> HHHHHHVPYSSAQSTSKTSVTLSLGGGTHADSLNNLANIKREQGNIEEAVRLYRKALEVFPEFAAAHSNLASVLQQQGKLQEALMHYKEAIRISPTFADAYSNMGNTLKEMQDVQGALQCYTRAIQINPAFADAHSNLASIHKDSGNIPEAIASYRTALKLKPDFPDAYCNLAHCLQIVCDWTDYDERMKKLVSIVADQLEKNRLPSVHPHHSMLYPLSHGFRKAIAERHGNLCLDKINVLHKPPYEHPKDLKLSDGRLRVGYVSSDFGNHPTSHLMQSIPGMHNPDKFEVFCYALSPDDGTNFRVKVMAEANHFIDLSQIPCNGKAADRIHQDGIHILVNMNGYTKGARNELFALRPAPIQAMWLGYPGTSGALFMDYIITDQETSPAEVAEQYSEKLAYMPHTFFIGDHANMFPHLKKKAVIDFKSNGHIYDNRIVLNGIDLKAFLDSLPDVKIVKMKCPDGGDNADSSNTALNMPVIPMNTIAEAVIEMINRGQIQITINGFSISNGLATTQINNKAATGEEVPRTIIVTTRSQYGLPEDAIVYCNFNQLYKIDPSTLQMWANILKRVPNSVLWLLRFPAVGE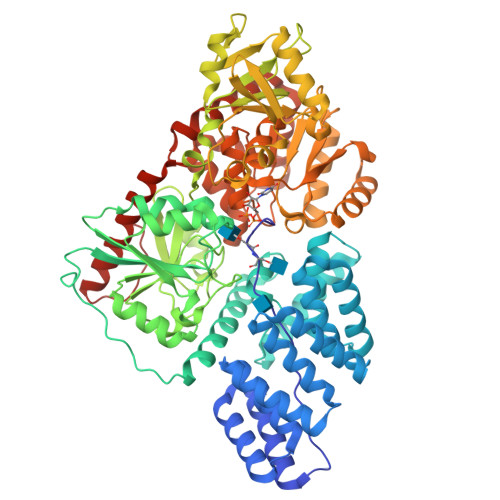PNIQQYAQNMGLPQNRIIFSPVAPKEEHVRRGQLADVCLDTPLCNGHTTGMDVLWAGTPMVTMPGETLASRVAASQLTCLGCLELIAKNRQEYEDIAVKLGTDLEYLKKVRGKVWKQRISSPLFNTKQYTMELERLYLQMWEHYAAGNKPDHMIKPVEVTESA> GMLSLAVNGTSQFTCFYNSRANISCVWSQDGALQDTSCQVHAWPDRRRWNQTCELLPVSQASWACNLILGAPDSQKLTTVDIVTLRVLCREGVRWRVMAIQDFKPFENLRLMAPISLQVVHVETHRCNISWEISQASHYFERHLEFEARTLSPGHTWEEAPLLTLKQKQEWICLETLTPDTQYEFQVRVKPLQGEFTT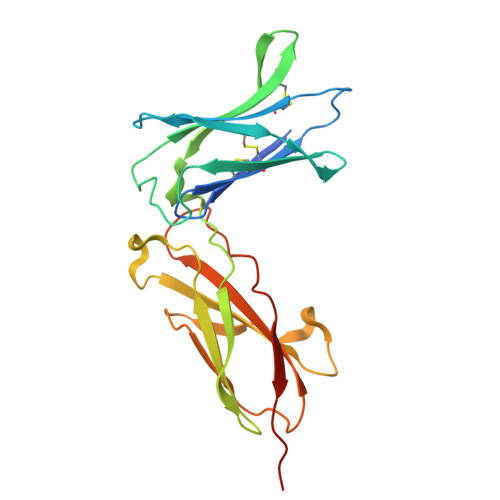WSPWSQPLAFRTKTGHHHHHH> GHM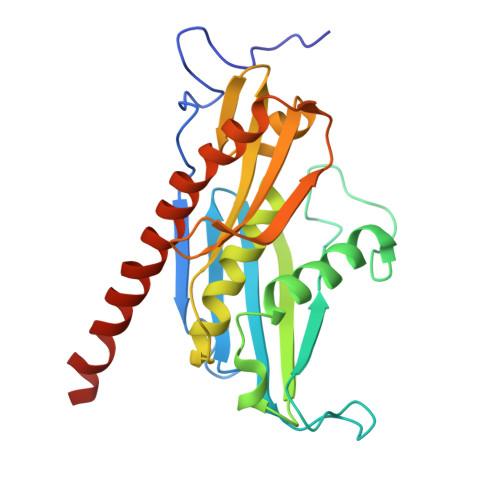SRLEIYSPEGLRLDGRRWNELRRFESSINTHPHAADGSSYMEQGNNKIITLVKGPKEPRLKSQMDTSKALLNVSVNITKFSKFERSKSSHKNERRVLEIQTSLVRMFEKNVMLNIYPRTVIDIEIHVLEQDGGIMGSLINGITLALIDAGISMFDYISGISVGLYDTTPLLDTNSLEENAMSTVTLGVVGKSEKLSLLLVEDKIPLDRLENVLAIGIAGAHRVRDLMDEELRKHAQKRVSNASAR To date, family GH139 is the only family known to be able to degrade α1,2-linked MeFuc, making it essential for RG-II metabolism and a feature of RG-II-degrading bacteria. In this report, we present the 3D structure of BT0984GH139, alongside its homolog SDT91673.1GH139 from Verrucomicrobium sp. GAS474, an organism isolated from forest soil. Crystals of BT0984GH139 formed in space group P212121 and diffracted to a resolution of 2.7 Å, while crystals of SDT91673.1GH139 formed in space group P 6522 and diffracted to 2.05 Å, providing good quality electron density maps in both cases. Both proteins adopt a three-domain architecture, consisting of an N-terminal β-sheet domain leading into an α-helical domain composed of a core (α/α)6 toroid structure. GH139 enzymes operate via an inverting mechanism in which we propose that N412 functions as the catalytic base and E561 acts as the catalytic acid (BT0984GH139 numbering).

To test whether an ortholog of BT0984GH139 from a soil environment was also an exo-acting 2-O-methyl-α-L-fucosidase, we cloned and recombinantly expressed, in Escherichia coli, SDT91673.1GH139 from Verrucomicrobium sp. GAS474; an organism isolated from a forest in Harvard, USA. However, SDT91673.1GH139 showed no detectable activity on any of the substrates tested. A glycerol molecule from the cryoprotectant occupies the suspected −1 subsite in SDT91673.1GH139, stacking against Trp686 and positioned above N412 and Q411. The SDT91673.1GH139 pocket is substantially more open and exhibits less hydrophobicity compared to BT0984GH139. The openness of the SDT91673.1GH139 pocket is facilitated by residues T462, T551, A487, and D473, which replace Q461, E561, W403, and E472 in BT0984GH139. In contrast, these residues are absent in SDT91673.1GH139. Specifically, W162 and W490 are spatially replaced by R189 and R186, respectively, introducing a more positively charged character. In SDT91673.1GH139, one of the rare (<1%) GH139 sequences that lacks the proposed catalytic acid, E561 (BT0984GH139 numbering), this position is instead occupied by T551. Interestingly, SDT91673.1GH139 belongs to the ∼1% of GH139 sequences that lack a catalytic acid residue, suggesting it may not serve an enzymatic role in Verrucomicrobium sp. GAS474 from which it was isolated, but instead may act as a glycan-binding protein for a substrate distinct from chain B of RG-II.

> SGAYDVTWDSVAWKNSAAKPWLGSMPLGNGDLGLNVWVEENGDLVFLIGKTDAWSENGELLKLGRVRLHLAASPLVAKSFRQVLKPEEGAVEVYSPADAPRPLYRVWVDANHPVAHVEVRTASGKATGAQADLELWRNEPREVRRVKGRERDNVEFNDGFRELRDTPGSLVTVDPDTVLPAKPGGDRIAWCHHNGRSLYPALLANQHLESLLPKYPDPLLNRTFGAVLEGPGFVASGDRTLKLMKESAAFRLDLYALATTAPDVEAWADDAGVLADTLSGLDIEAARLAHRNWWRAFWGRSWIVVDGNDLPGGDPTDGEMARAVTQSYAMQRWMTAGSGRSVAAMPIPFNGAIFTVGKETPKEKYDPAKGDTGNPDFRTGGGNIPFQNTRHIYWPMLASGDYDLMRPFFRRYRENLALLTERTRLYDKHAGAAFPETGFFWGLPNDADFGIGNKEAVLQNLAIRYEIQGGLELTAMMLDYYDATQDTDFLVNTLLPLADGVAAYYDQHWQRGGDGKIVFSPAQSLTTYQSPSGKDVVNPLPDIAGLMAVLPRLIALPPGTATAAQRTAWKKTLADLPPLPRGKTGTGRNNTPDKVPIPSTTQKDDGAPILLPAQVYGTEKNVENPEEYAIFPYRLFGVGLPEIDLGLNTFRARNFTDSTGWAWDGIVAACLGLSDDAKREAIRNFAEDRNPDTGHGPNYPGLSAFSREARFKWFWKPGPSSGPGNGTEPALDNGGVGQSILQSMLLQQRGEKIVLFPAWPKEWNVSFKLHAARNTTVEGVLKNGKLERLTVTPPERRGDVIVREAQ>AAPQQINDIVHRTITPLIEQQKIPGMAVAVIYQGKPYYFTWGYADIAKKQPVTQQTLFELGSVSKTFTGVLGGDAIARGEIKLSDPTTKYWPELTAKQWNGITLLHLATYTAGGLPLQVPDEVKSSSDLLRFYQNWQPAWAPGTQRLYANSSIGLFGALAVKPSGLSFEQAMKTRVFQPLKLNHTWINVPSAEEKNYAWGYREGKAVHVSPGALDAEAYGVKSTIEDMARWVQSNLKPLDINEKTLQQGIQLAQSRYWQTGDMYQGLGWEMLDWPVNPDIIINGSDNKIALAARPVKPITPPTPAVRASWV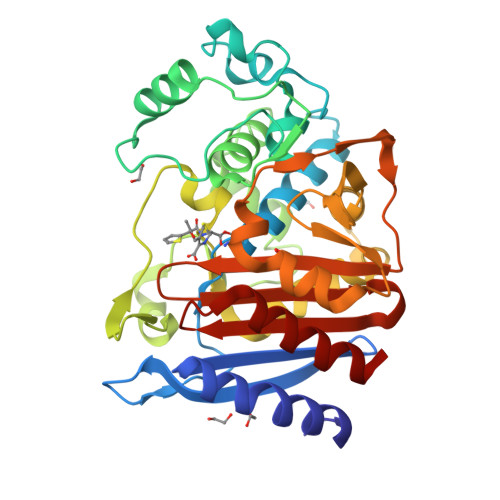HKTGATGGFGSYVAFIPEKELGIVMLANKNYPNPARVAAAWQILNALQ[2x]>[4x]GAMEPKASCPAAAPLMERKFHVLVGVTGSVAALKLPLLVSKLLDIPGLEVAVVTTERAKHFYSPQDI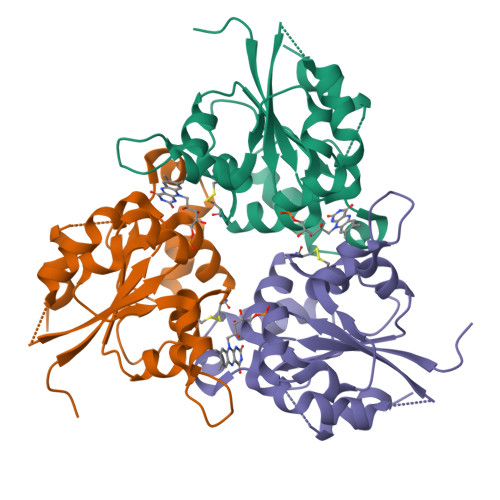PVTLYSDADEWEMWKSRSDPVLHIDLRRWADLLLVAPLDANTLGKVASGICDNLLTCVMRAWDRSKPLLFCPAMNTAMWEHPITAQQVDQLKAFGYVEIPCVAKKLVCGDEGLGAMAEVGTIVDKVKEVLFQHSGFQQS> SRHS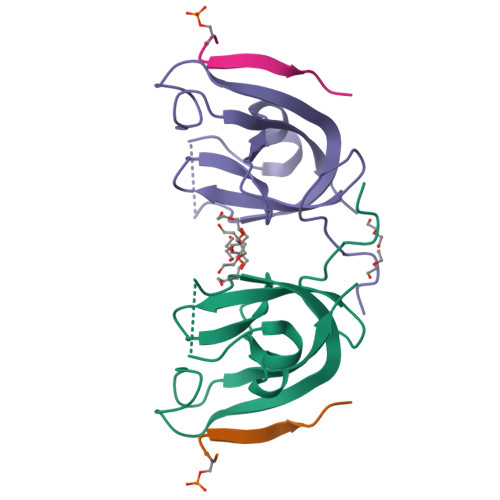EKIAIRDFQVGDLVLIILDERHDNYVLFTVSPTLYFLHSESLPALDLKPGEGASGASRRPWVLGKVMEKEYCQAKKAQNRFKVPLGTKFYRVKAVSWNKKV;> SDDSDIVTLEPPK> MNLFWPSETKKQNEIPGGDYTPGNSPSVQKGYQFLNRDIFKSCPRIMERQFGECLHNRTHLIKDLISSGNVGLGPIEIVHMSYLNKHEKEEFGEYFYVTGIEVSGPAMPVEFLEVLKSSKRISKNISNNIILTYCCFNFFSNLDIRIRYDADDTFQTTAIDCNKETTDLTMTEKMWEETFASSVIRAIITNTNPELKPPGLVECPFYVGKDTISSCKKIIELLCRFLPRSLNCGWDSTKSMQATIVNNYLMYSLKSFIAITPSLVDFTIDYLKGLTKKDPIHDIYYKTAMITILDHIETKELDMITILNETLDPLLS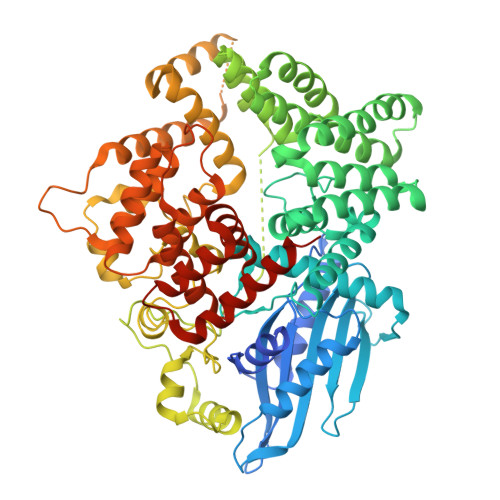LLNDLPPRDADSARLMNCMSDLLNIQTNFLLNRGDYELALGVSNTSTELALDSFESWYNLARCHIKKEEYEKALFAINSMPRLRKNDGHLETMYSRFLTSNYYKKPLNGTREHYDLTAMEFTNLSGTLRNWKEDELKRQIFGRIAMINEKKIGYTKEIWDDIAIKLGPICGPQSVNLINYVSPQEVKNIKNINLIARNTIGKQLGWFSGKIYGLLMEIVNKIGWNGLLNIRTEAFMMETEFYQASNNIIDENGHIPMESRKKRFCEGWLDDLFLDLYQDLKLSKISLSNKDEKHSGLEWELLGLIMLRTWHWEDAVACLRTSIVARFDPVSCQQLLKIYLQPPKNIQEVTLLDTDTIISLLIKKISYDCRYYNYCQIFNLQLLEKLCNELGTHILRNKILLQPSIGDEIMVMIDAMLAWIADLDHTVQPGTENLYFQ> MAEKFDHLEEHLEKFVENIRQLGIIVSDFQPSSQAGLNQKLNFIVTGLQDIDKCRQQLHDITVPLEVFEYIDQGRNPQLYTKECLERALAKNEQVKGKIDTMKKFKSLLIQELSKVFPEDMAKYRS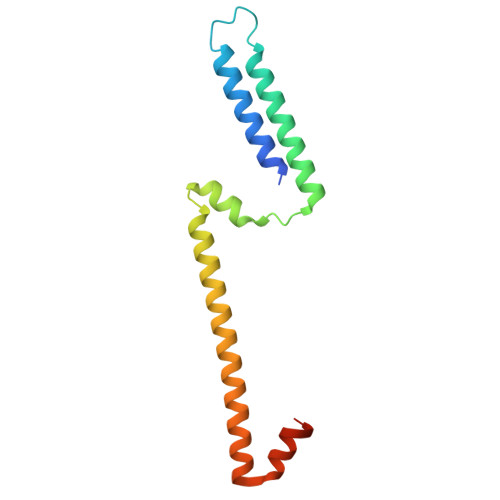IRGEDHPPS>MAQVLIVGAGMTGSLCAALLRRQTSGPLYLAVWDKADDSGGRMTTACSPHNPQCTADLGAQYITCTPHYAKKHQRFYDELLAYGVLRPLSSPIEGMVMKEGDCNFVAPQGISSIIKHYLKESGAEVYFRHRVTQINLRDDKWEVSKQTGSPEQFDLIVLTMPVPEILQLQGDITTLISECQRQQLEAVSYSSRYALGLF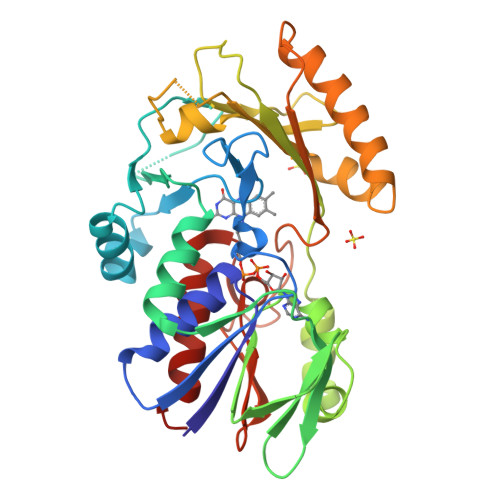YEAGTKIDVPWAGQYITSNPCIRFVSIDNKKRNIESSEIGPSLVIHTTVPFGVTYLEHSIEDVQELVFQQLENILPGLPQPIATKCQKWRHSQVTNAAANCPGQMTLHHKPFLACGGDGFTQSNFDGCITSALCVLEALKNYI[2x]In coumarin biosynthesis, a BAHD acyltransferase-family enzyme COSY was recently discovered to accelerate coumarin formation as the only known BAHD enzyme to catalyze an intramolecular acyl transfer reaction. To understand the mechanistic basis for the unconventional activity of COSY as a BAHD-family enzyme, we present several crystal structures of A. thaliana COSY (AtCOSY) in its apo and various ligand-bound forms. The AtCOSY active site is located at the interface between the two pseudo-symmetric domains, and features the conserved catalytic residues, His161 and Trp371, stemming from the N- and C-terminal domains, respectively.

To investigate the molecular basis for the unique catalytic activity of COSY, we first obtained the apo structure of AtCOSY at 1.9 Å resolution. Additionally, we observed a single Ca2+ ion that binds to the linker loop region and is coordinated by the main-chain carbonyl oxygens of Arg211 and Leu214 residues. Since we observed binding of a Ca2+ ion in the AtCOSY structure, we tested whether the coumarin synthase activity may be dependent upon Ca2+ or other divalent metals. Nevertheless, we observed no significant difference in coumarin synthase activity whether or not Ca2+ is present in the assay buffer. Similarly, addition of Zn2+, Ni2+, Mn2+, Co2+, Fe2+ or Cu2+ to the assay buffer had little impact on the coumarin synthase activity, suggesting the observed calcium-binding site may be an artifact of crystallization. We noticed a similar backbone fold and consistent positioning of most of the active-site-lining residues in these predicted structures compared to the solved apo-structure of AtCOSY.

>MATLEITDIALVQPSHQPLSNDQTLSLSHLDNDNNLHVSFRYLRVYSSSSSTVAGESPSAVVSASLATALVHYYPLAGSLRRSASDNRFELLCSAGQSVPLVNATVNCTLESVGYLDGPDPGFVERLVPDPTREEGMVNPCILQVTMFQCGGWVLGASIHHAICDGLGASLFFNAMAELARGATKISIEPVWDRERLLGPREKPWVGAPVRDFLSLDKDFDPYGQAIGDVKRDCFFVTDDSLDQLKAQLLEKSGLNFTTFEALGAYIWRAKVRAAKTEEKENVKFVYSINIRRLMNPPLPKGYWGNGCVPMYAQIKAGELIEQPIWKTAELIKQSKSNTSDEYVRSFIDFQELHHKDGINAGTGVTGFTDWRYLGHSTIDFGWGGPVTVLPLSNKLLGSMEPCFFLPYSTDAAAGSKKDSGFKVLVNLRESAMPEFKEAMDKFHKGEFALS[2x]> MSPIIEANGTLDELTSFIGEAKHYVDEEMKGILEEIQNDIYKIMGEIGSKGKIEG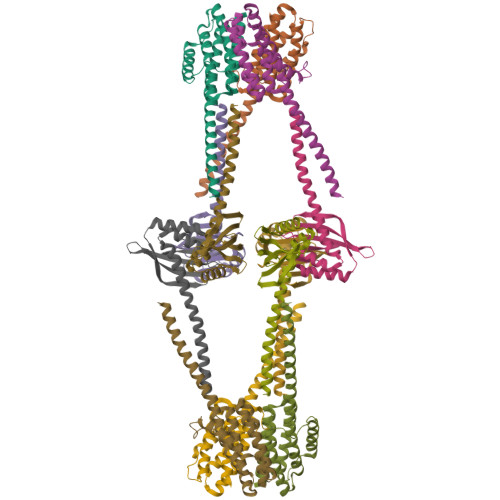ISEERIKWLEGLISRYEEMVNLKSFVLPGGTLESAKLDVCRTIARRAERKVATVLREFGIGKEALVYLNRLSDLLFLLARVIEIAAAAQLEKELQALEKENAQLEWELQALEKELAQ;> MAQLKKKLQALKKKNAQLKWKLQALKKKLAQATQHLTIAQTYLAAWNEEDNERRRHLVGQAWAENTRYVDPLMQGEGQQGIAAMIEAARQKFPGYRFVLAGTPDGHGNFTRFSWRLISPDGDDVAGGTDVVSLNTEGRIDNVVGFLDGAVSHHHHHH>[2x]GSMAQEAGSCVQDGQRYNDKDVWKPEPCRICVCDTGTVLCDDIICEDVKD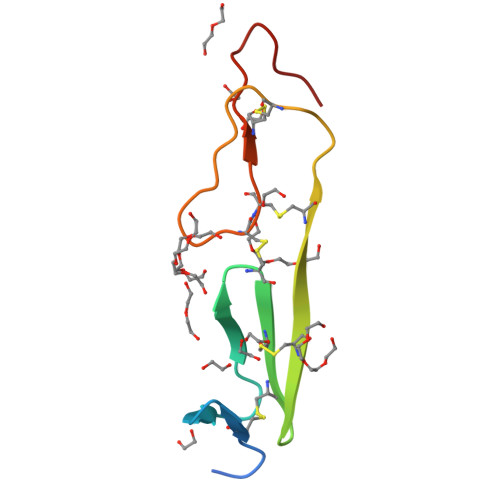CLSPEIPFGECCPICPTDLATASG> SPTVEECGYSDRARSITLGNSTITTQECANVVVGYGVWPDYLKDSEATAED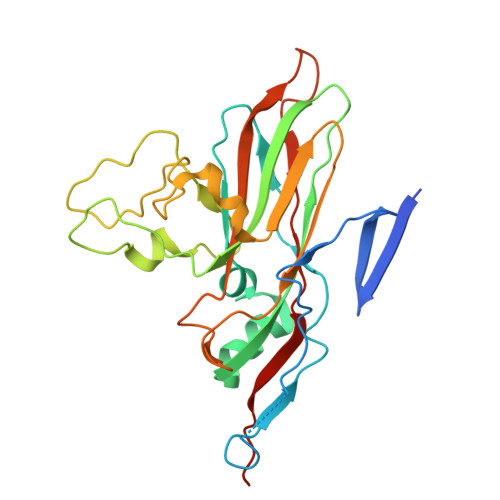QPTQPDVATCRFYTLDSVQWQKTSPGWWWKLPDALSNLGLFGQNMQYHYLGRTGYTVHVQCNASKFHQGCLLVVCVPEAEMGCATLDNTPSSAELLGGDSAKEFADKPVASGSNKLVQRVVYNAGMGVGVGNLTIFPHQWINLRTNNSATIVMPYTNSVPMDNMFRHNNVTLMVIPFVPLDYCPGSTTYVPITVTIAPMCAEYNGLRLAGHQ> SLFEAWAKPVQPFAIWPGVWYVGTENLSSVLLTTPQGHILIDAGLDASAPQIRRNIEALGFRMADIRYIANSHAHLDHAGGIARLKAWSGARVIASHANAEQMARGGKEDFALGDALPFP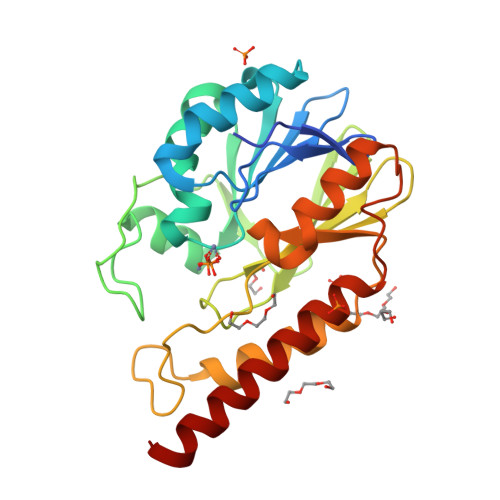PVTVDMEAQDGQQWHLGGVTLAAIFTPGHLPGATSWKVTLADGKTLIYADSLATPGYPLINNRNYPTLVEDIRRSFARLEAQQVDIFLANHGERFGLMDKMARKARGENNAFIDKAGLARYVAQSRAAFEKQLAAQRAQP> MKHLHRFFSSDASGGIILIIAAILAMIMANSGATSGWYHDFLETPVQLRVGSLEINKNMLLWINDALMAVFFLLVGLEVKRELMQGSLASLRQAAFPVIAAIGGMIVPTLLYLAFNYADPITREGWAIPAATDIAFALGVLALLGSRVPLALKIFLMALAIIDDLGAIIIIALFYTNDLSMASLGVAAVAIAVLAVLNLCGARRTGVYILVGVVLWTAVLKSGVHATLAGVIVGFFIPLKEKHGRSPAKRLEHVLHPWVAYLILPLFAFANAGVSLGGVTLDGLTSILPLGIIAGMLIGKPLGISLFCWLALRLKLAHLPEGTTYQQIMVVGILCGIGFTMSIFIASLAFGSVDPELINWAKLGILVGSISSAVIGYSWLRVRLRPSVGSENLYFQ

Na+/H+ antiporters are found in all cells to help regulate intracellular pH, sodium levels, and cell volume. Bacterial NhaA is an electrogenic Na+/H+ antiporter that transports 2 H+ in exchange for 1 Na+ across the membrane. The NhaA-fold consists of a scaffold domain that mediates dimerization (dimer domain), and an ion-translocation (core) domain, which is typified by a six transmembrane (TM) bundle harbouring two opposite-facing discontinuous helices that crossover near the centre of the membrane. EcNhaA is inactive below pH 6.0, and between pH 6.5 and pH 8 transport rates increase 2000-fold.

Here we determine the crystal structure of EcNhaA at active pH 6.5 at 2.2 Å resolution. The monoLCP-NhaA crystallized as a non-physiological monomer, like the previous mono-NhaA crystal structure determined at 3.45 Å resolution at inactive pH 412. In the NhaA crystal structure at active pH 6.5, Arg81 in TM2 breaks its salt-bridge interaction with Glu252 in TM9 and forms a tighter salt-bridge (>3.3 Å) to Glu78 located on its own helix, stabilized by Glu82 and Glu252 through interactions with Glu78. In particular, the rearrangement of Asp11 in TM1 has broken its interaction with His256 in TM9 and reformed a salt-bridge to Lys153 in TM5, which has also shifted its position. Since the ion-binding Asp164 is located on TM5, there is therefore a direct physical coupling between the pH induced changes and the ion-binding site. The concerted movement of Arg81, His256 and Asp11 side-chains at active pH has caused a dramatic widening of the intracellular funnel. Consistently, we find that only at active pH 6.5 is the intracellular funnel in NhaA wide enough to accommodate a hydrated Na+ ion to the ion-binding site, as assessed by HOLE analysis. In addition, 106 crystallographic waters were modelled with one of the waters in hydrogen bond distance to the ion-binding Asp163. We further show that the neighbouring Asp163 forms a salt-bridge to Lys300 at both inactive and active pH, but only at active pH do molecular dynamics (MD) simulations show that Na+ binding induces salt-bridge breakage, an essential step in the transport cycle. In contrast, under inactive pH conditions, the cytosolic funnel contracted over the course of the simulation with concomitant changes in salt bridge interactions, preventing Na+ access to the binding site. Taken together, we conclude the pH sensor is rather working as a pH gate, controlling access to the ion-binding site.Archaemetzincins are metalloproteases occurring in archaea and some mammalia. They are distinct from all the other metzincins by their extended active site consensus sequence HEXXHXXGXXHCX4CXMX17CXXC featuring four conserved cysteine residues. The overall structure of AfAmzA resembles those of other metzincins, consisting of an upper N-terminal domain (NTD) and a lower helical C-terminal domain (CTD) with respect to the active site helix α2, which harbors two of the three zinc-binding histidines (H117EIGH121) and the catalytic base Glu118. On the other hand, as the homologous archaemetzincins from Methanopyrus kandleri (MkAmzA) and Methanocorpusculum labreanum (MlAmzA), AfAmzA exhibits a second zinc-binding site located in the CTD immediately below the catalytic zinc binding site and close to the eponymous, structurally important Met-turn.

Consequently, two different crystal forms are observed, one triclinic and one hexagonal. In the nat-AfAmzA::malonate complex the catalytic zinc ion is coordinated in a tetrahedral geometry by the three histidine side-chains as well as by one carboxylate oxygen atom (O7) of malonate, with ligand-metal distances of 2.0–2.1 Å. The catalytic water molecule is displaced by the malonate O7 atom and is moved towards the catalytic base Glu118. While both nat-AfAmzA structures with carboxylic acids bound in the active-site cleft superpose quite well despite different crystal lattices, the structural superimposition of nat-AfAmzA::malonate with NHis-AfAmzA shows that substantial changes take place in the bulge edge segment and the S1′-wall forming segments, effecting main-chain and side-chains of the corresponding residues. This is opening up the substrate-binding groove in order to provide space for a ligand. The side-chains of the conserved Phe80 and Phe82 residues move slightly while the side chain of Met78 adopts another conformation. In the S1′-wall forming segment the side chain of Phe136 performs a χ1 rotation of 115° and interacts with the malonate carboxylate group with its Cδ1 just 3.3 Å away from the malonate oxygen atom. The side chain of Asn138 follows this movement by occupying another rotamer while its main chain Cα moves by 2.1 Å. On the other hand, we detect upon ligand binding opening of the active site at the S' sites.

>MKIYIQPLSVNSHTVEVLANSLPKIFNAEVFVLPASDVSLKCYNASRRQYNSTCILRMLPPIKVTLGVTGKDIYAKGMNFVFGEAELGGARAVLSVFRLTTADSELYRERVVKEAVHEIGHVLGLKHCSNNCVMRFSNSVQDVDRKPVSFCRECASKIRY[3x]> MNYPVNPDL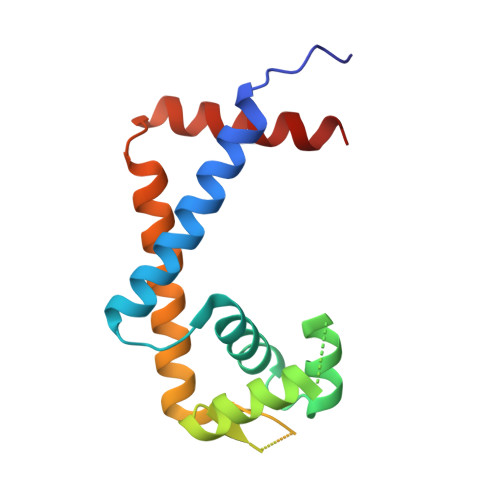MPALMAVFQHVRTRIQSELDCQRLDLTPPDVHVLKLIDEQRGLNLQDLGRQMCRDKALITRKIRELEGRNLVRRERNPSDQRSFQLFLTDEGLAIHLHAELIMSRVHDELFAPLTPVEQATLVHLLDQCLAAQ> GTTVHCDYLNRPHKSIHRRRTDPMVTLSSILESIINDMRDLPNTYPFHTPVNAKVVKDYYKIITRPMDLQTLRENVRKRLYPSREEFREHLELIVKNSATYNGPKHSLTQISQSMLDLCDEKLKEKEDKLARLEKAINPLLDDDDQVAFSFILDNIVTQKMMAVPDSWPFHHPVNKKFVPDYYKVIVNPMDLETIRKNISKHKYQSRESFLDDVNLILANSVKYNGPESQYTKTAQEIVNVCYQTLTEYDEHLTQLEKDICTAKEAALEEAEL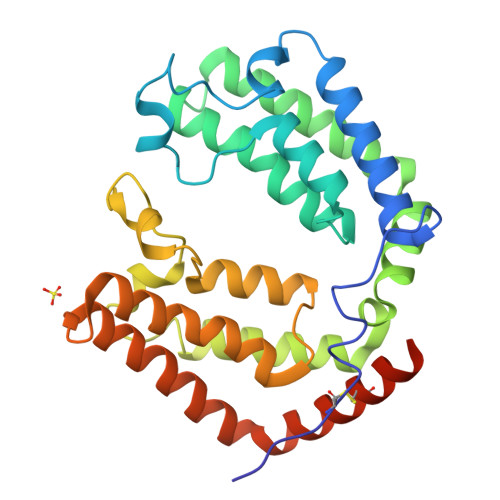ESLDPMT> CGUGGUUGACACGCAGACCUCUUACAAGAGUGUCUAGGUGCCUUUGAGAGUUACUCUUUGCUCUCUUCGGAAGAACCCUUAGGGGUUCGUGCAUGGGCUUGCAUAGCAAGU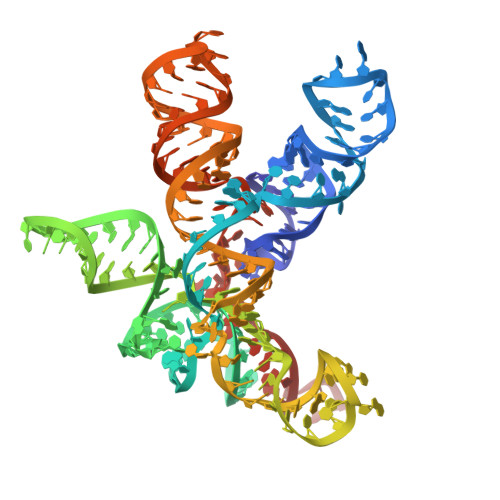CUUAGAAUGCGGGUACCGUACAGUGUUGAAAAACACUGUAAAUCUCUAAAAGAGACCA>MGSAMSLGCSKRKATNQDVDSESRKRRKICSTNDAENCRFIQDESSWKHPWSLCANSVVNDTKDTKSSALSLPSPPTSVSRIWKHQVFPSFHGADVRKTILSHILESFRRKGIDPFIDNNIERSKSIGHELKEAIKGSKIAIVLLSKNYASSSWCLDELAEIMKCRELLGQIVMTIFYEVDPTDIKKQTGEFGKAFTKTCKGKTKEYVERWRKALEDVATIAGYHSHKWRNEADMIEKIATDVSNMLNSFKPSRDFNGLVGMRAHMDMLEQLLRLVLDEVRMIGIWGPPGIGKTTIARFLFNQVSDRFQLSAIMVNIKGCYPRPCFDEYSAQLQLQNQMLSQMINHKDIMISHLGVAQERLRDKKVFLVLDEVDQLGQLDALAKETRWF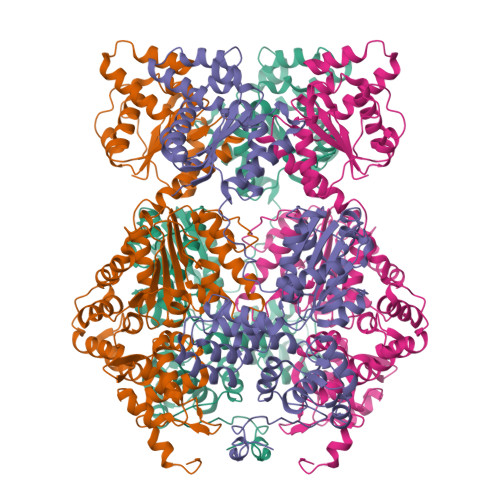GPGSRIIITTEDLGVLKAHGINHVYKVGYPSNDEAFQIFCMNAFGQKQPHEGFDEIAREVMALAGELPLGLKVLGSALRGKSKPEWERTLPRLKTSLDGKIGSIIQFSYDALCDEDKYLFLYIACLFNKESTTKVEGLLGKFLDVRQGLHILAQKSLISIEDGNIYMHTLLEQFGRETSRKQFIHHGYTKHQLLVGERDICEVLNDDTIDSRRFIGINLDLYKNVEELNISEKALERIHDFQFVRINGKNHALHERLQGLIYQSPQIRSLHWKCYQNICLPSTFNSEFLVELDMSFSKLQKLWEGTKQLRNLKWMDLSYSSYLKELPNLSTATNLEELKLRNCSSLVELPSSIEKLTSLQILDLHRCSSLVELPSFGNATKLEILNLENCSSLVKLPPSINANNLQELSLTNCSRVVELPAIENATNLWKLNLLNCSSLIELPLSIGTATNLKHLDFRGCSSLVKLPSSIGDMTNLEVFYLSNCSNLVELPSSIGNLRKLTLLLMRGCSKLETLPTNINLKSLHTLNLIDCSRLKSFPEISTHIKYLRLIGTAIKEVPLSIMSWSPLAHFQISYFESLKEFPHALDIITELQLSKDIQEVPPWVKRMSRLRALRLNNCNNLVSLPQLPDSLAYLYADNCKSLERLDCCFNNPEIRLYFPKCFKLNQEARDLIMHTSTRNFAMLPGTQVPACFNHRATSGDSLKIKLKESPLPTTLTFKACIMLVNEEMSYDLKSMSVDIVIRDEQNDLKVQCTPSYHQCTEIYVLTEHIYTFELEVEEVTSTELVFEFTSVNESICKIGECGILQRETRSLRRSSSPDLSPESSRVSSCDHC[4x]>[4x]MKLKHKRDDKMRFDIKKVLELAEKDFETAWRETRALIKDKHIDNKYPRLKPVYGKPHPVMETIERLRQ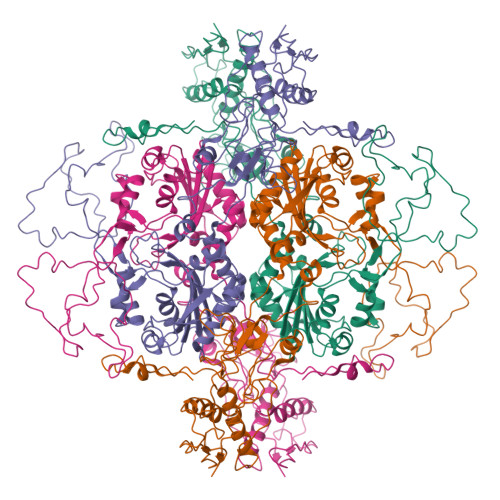AYLRMGFEEMINPVIVDEMEIYKQFGPEAMAVLDRCFYLAGLPRPDVGLGNEKVEIIKNLGIDIDEEKKERLREVLHLYKKGAIDGDDLVFEIAKALNVSNEMGLKVLETAFPEFKDLKPESTTLTLRSHMTSGWFITLSSLIKKRKLPLKLFSIDRCFRREQREDRSHLMSYHSASCVVVGEDVSVDDGKVVAEGLLAQFGFTKFKFKPDEKKSKYYTPETQTEVYAYHPKLGEWIEVATFGVYSPIALAKYNIDVPVMNLGLGVERLAMIIYGYEDVRAMVYPQFYEYRLSDRDIAGMIRVDKVPILDEFYNFANELIDICIANKDKESPCSVEVKREFNFNGERRVIKVEIFENEPNKKLLGPSVLNEVYVYDGNIYGIPPTFEGVKEQYIPILKKAKEEGVSTNIRYIDGIIYKLVAKIEEALVSNVDEFKFRVPIVRSLSDINLKIDELALKQIMGENKVIDVRGPVFLNAKVEIK>[4x]MIKVRVPDFSDKKFSDRWRYCVGTGRLGLALQKEYIETLKYVKENIDFKYIRGHGLLCDDVGIYREDVVGDEVKPFYNFTYIDRIFDSFLEIGIRPFVEIGFMPKKLASGTQTVFYWEGNVTPPKDYEKWSDLVKAVLHHFISRYGIEEVLKWPFEIWNEPNLKEFWKDADEKEYFKLYKVTAKAIKEVNENLKVGGPAICGGADYWIEDFLNFCYEENVPVDFVSRHAYTSKQGEYT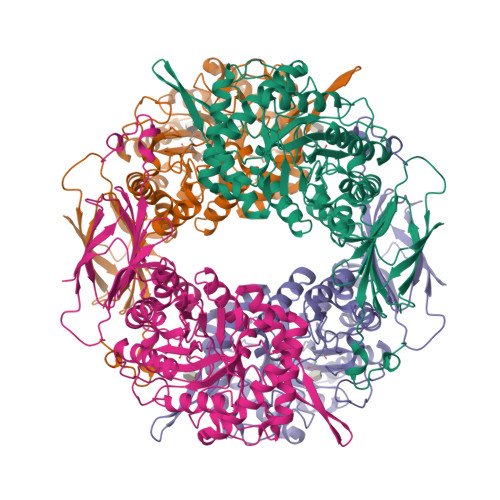PHLIYQEIMPSEYMLNEFKTVREIIKNSHFPNLPFHITEYNTSYSPQNPVHDTPFNAAYIARILSEGGDYVDSFSYWTFSDVFEERDVPRSQFHGGFGLVALNMIPKPTFYTFKFFNAMGEEMLYRDEHMLVTRRDDGSVALIAWNEVMDKTENPDEDYEVEIPVRFRDVFIKRQLIDEEHGNPWGTWIHMGRPRYPSKEQVNTLREVAKPEIMTSQPVANDGYLNLKFKLGKNAVVLYELTERIDESSTYIGLDDSKINGY We isolated and characterized two Shigella podophages that have notably different features when compared with classical podophages and instead are most closely related to phage N4. We describe the isolation and characterization of phages Moo19 and B2, including whole-genome sequencing and analysis, cryo–electron microscopy (cryo-EM) structure determination, mass spectrometry, host range studies, and enzymatic assays of the tail proteins. Our work shows that these phages have divergent decoration proteins and unique tail structures, and encode and package their own phage-dependent RNA polymerase, and the tails, which display esterase activity, are dependent on specific O-antigen modifications of lipopolysaccharide (LPS) for entry. Moo19 and B2 are similar to bacteriophage N4—these are all T = 9 podophages, which encapsidate their own polymerases—a hallmark of this phage family.

Because we could not resolve the highly flexible side tailspikes in either Moo19 or B2 virions, we purified these components to examine them separately. Genome analysis and mass spectrometry data indicated that the tailspike was a single protein in Moo19 (gp82) and a complex of two proteins in B2 (gp48/gp49). We used a similar approach as described by Subramanian et al. and purified gp82 alone. We also copurified a complex of gp48/gp49 as previously described. Using cryo-EM, we solved the structure of the isolated tailspikes to 2.4- and 2.3-Å resolution, respectively. The tailspikes most closely resemble that of the tailspike in phage G7C and differ wildly from the tailspikes in DEV, which more closely resemble a myophage fiber. Each structure is a homotrimer, with individual ribbons colored cyan, green, and magenta. Therefore, we tested the purified Moo19 tailspike gp82 and the complex tailspike from B2, gp49/49, for esterase activity using a colorimetric assay. Positive esterase activity would result in a visibly yellow color and increased absorbance with time. Both tailspikes exhibited a rapid, dose-dependent color change, indicating esterase activity. In G7C, this appendage is hypothesized to expand the host range; however, Moo19 and B2 have the same host range, so the function of gp81 in Moo19 is unclear at this time. Three major structural differences (see cartoon representation in Fig. 3B) include (i) the lack of the tail appendage, (ii) a single tailspike for Moo19 and a complex of two proteins for B2 (see next two paragraphs), and (iii) the completely different decoration proteins.

> MNQLFSQGGKGSAGILTNKQAVARHFGVKQSEVVYFSVGVDISGYKVIYDKTTQRAYSLPIGIPAGTTAISLSTAAVLVHSQGSVDLGAVAVLRKEYVTIPGDFTSGATIQVKNEILTHSNGAQYRWAGAVPKVVPAGSTPASSGGISASAWIEVTGEELRDELATTGGASQIGTSDGKTVQQWIIANDSANYRARNIQKLAWVDKQVHSRGSIKVLFQGDSMTAGYDTTSTDRVPANNGDWATHASMTYPQRFMAYLPEQSGCSVTGVYRAISGHTAIQSYNEPSWQSNPNCDVVILMLGLNDAGGVAGTTEDIYMEYMEKLIRRFIDWGMGVVVQTCSTGGQGSGGVVANLWAKRMRMMADTYGCAHFNADEVQYYRHNGAVQSDGGHFNSMGYAIHGQMLASMFMAGGLLPTYRPLTNEINTWCGRLDDSIGYCDATGNINLGRSDGAYTRTKVVGGMLANVASIATFSFYLDAEAAHIFVHGSGAGPINVLVDAPSWWNNGAQDYYDFANNQSINFSNSPQAANNAIVDLSTTYSADRKFVGRILGRGWKTLTFFTNLQGTGGDFYLNSLTVQPVPVGMSVQARNWARFDKGHRAVYSKKIPQAYNQATLPTATALVNFQVPMPQSMLPTTPSISGDLGTNFYNCGHSVLKISNSSGDYLEVLLIKTTGGGYVFTGKILKTTYATGNQPTAITATAAHYSMKDLKVAGANGPNMPLETIRDIDMASYVTIGVGAGNGGLVLDINITWPSTPPTSYWNIELEAWDMFGNSEASI;> MIRTTNTCCGNQAGMVEKFIGTAYDVVKTVYDNLGEIQFIYNFLNDYGVLITVDSVTELQELPTTAKYTRVYSSTPTGVRIYTDYLYVEGDRTGVLPSDPTATGSWVVVGSSNSGAATGTGAYIPFVFNNGSAAGGETTIVVPDYTIGVPEIYVEGFRQQVGRGFTFNSVNLTVTLAQPLEQGDEVVLMLSGNPAVPDNPNIDSWTVINWIYNNGAAVGGEQVIVIPYTFQTVPAIFKNGLRYQGGLSTQSYTVDQDNKRILLTEPLSTNDRLVVQLGGELVTLESPDRSLYEIARATNMKDSEVIKSDNTVETLNGKRILYDIVSQVYYWIPSSVPNNVYIQSVVNGQLTYLPGNIVVTLTPIVTLGLSGTTAQRPIGVLTGTQHFDTTLGKPIWFNGTAWVDSTGAVV>[6x]MGSSHHHHHHHSSGLVPRGSHMDPVSVWGNTPLATVDPEIHDLIEKEKRRQCRGIELIASENFTSFAVIEAL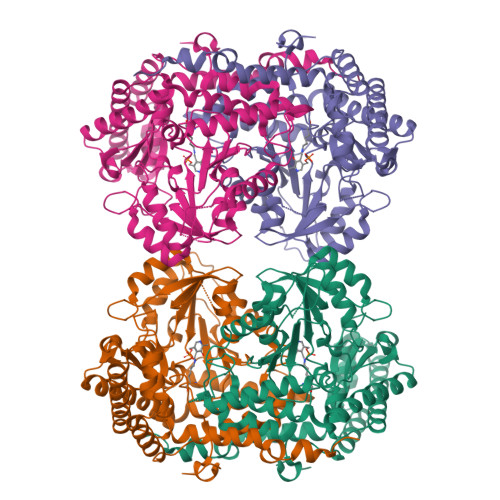GSALTNKYSEGMPGNRYYGGNEYIDQIENLCRSRALQAFHLDAQSWGVNVQPYSGSPANFAAYTAVLNPHDRIMGLDLRSGGHLTHGYYTSGGKKISATSIYFESLPYKVNSTTGYIDYDRLEEKALDFRPKLIICGGSAYPRDWDYKRFREVADKCGALLLCDMAHTSGLVAAQEVNSPFEYCDIVTTTTHKSLRGPRAGMIFYRKGPKPPKKGQPENAVYDFEDKINFAVFSSLQGGPHNHQIGALAVALKQAASPGFKAYAKQVKANAVALGKYLMGKGYSLVTGGTENHLVLWDLRPLGLTGYKVEKLCDLCNITVNKNAVFGDSSALAPGGVRIGAPAMTSRGLVEKDFEQIGEFLHRAVTLTLEIQKEHGKLLKDFNKGLVNNKAIEDLKADVEKFSALFDMPGFLVSEMKYKD>HHHHHHHHENLYFQGDPTQFEERHLKFLQQLGKGNFGSVEMCRYDPLQDNTGEVVAVKKLQHSTEEHLRDFEREIEILKSLQHDNIVKYKGVCYSAGRRNLKLIMEYLPYGSLRDYLQKHKERIDHIKLLQYTSQICKGMEYLGTKRYIHRDLATRNILVENENRVKIGDFGLTKVLPQDKEYYKVKEPGESPIFWYAPESLTESKFSVASDVWSFGVVLYELFTYIEKSKSPPAEFMRMIGNDKQGQMIVFHLIELLKNNGRLPRPDGCPDEIYMIMTECWNNNVNQRPSFRDLALRVDQIRDNMAG[2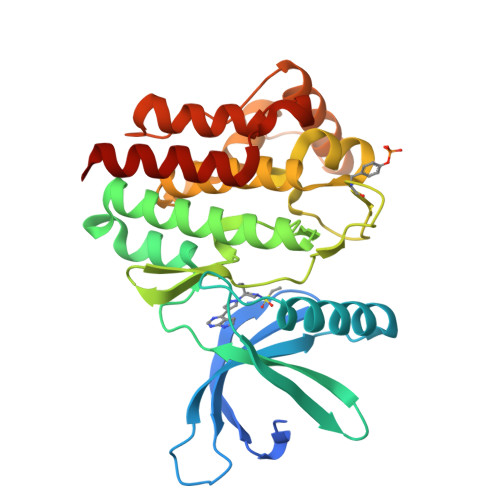x]The 26S proteasome is a 2.5 MDa protease dedicated to the degradation of ubiquitinated proteins in eukaryotes. The RP-specific chaperones Nas6, Nas2, Hsm3 and Rpn14 are important for the assembly of a hetero-hexameric AAA-ATPase ring formed by the subunits Rpt1 to Rpt6. One of these, Nas2, binds to the proteasomal AAA-ATPase subunit Rpt5. The PDZ domain of Nas2 binds to the C-terminal tail of Rpt5; however, it does not require the C-terminus of Rpt5 for binding.

Since no crystals were obtained, we created two truncated forms of Nas2 with the goal of minimizing the sequence around the PDZ domain. Nas2LND produced well diffracting crystals after two months, enabling us to determine a structure comprised of amino acids Gln129–Leu220 in the asymmetric unit. Nas2LND adopts a fold consisting of five β-sheets and two α-helices commonly found amongst PDZ-domain structures. N-terminal residues from cloning that spanned Gly115–Gly124 could be traced in the electron-density maps. However, residues between Gly124 and Gly129 were disordered and could not be modeled. Following refinement, recurring electron density was observed in two regions. The first was modeled as a disordered PEG 400 fragment obtained from the cryoprotectant. Nas2 lacks the GLGF motif commonly found just prior to β-strand 2 in PDZ domains. The absence is not surprising as the Nas2 structure shows that β-strand 5, instead of the common β-strand 2, contributes to the putative peptide-binding groove, causing a different loop arrangement. The reported Nas2 structure will provide the basis for further insights regarding the structure and function of Nas2 in proteasome assembly, as it will facilitate molecular docking of the tail of Rpt5 as well as enabling the design of Nas2 mutants based on the putative binding region.

> GPLTRRASVGSQAIQYTIPFAFISEVVPGSPSDKADIKVDDKLISIGNVHAANHSKLQNIQMVVMKNEDRPLPVLLLREGQILKTSLTPSRNWNGRGLLGCRIQEL> ARIKAINTF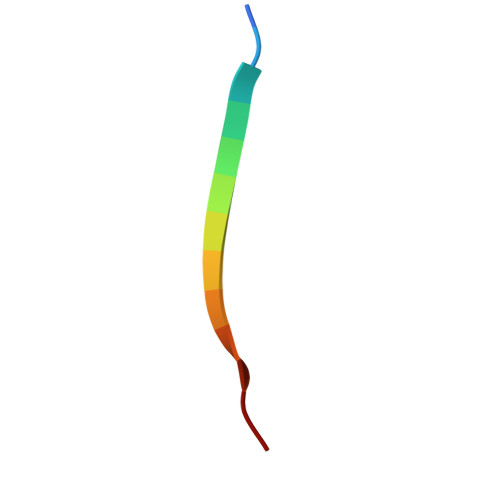FAKN>MTNQYSVKPQLVMFTGGRDSTLAACYLMLQGIPVHLWSGNSGCSLHRGILSHRVEEMKNRFGDLVVGHTVADISGAFRSIAIEALEQDILKYRKNLVLLGEKLAIHAHLVDFCRRNDINTINDGITHYQMEFPEQRLVAKTFLMEMMAQYDINYQSPVYEFAQSADDVKYRLLQLGISTKSLEGISIFADSFSTPSDDVVLAYLREKAPLAHNIVNFLAGETLNPP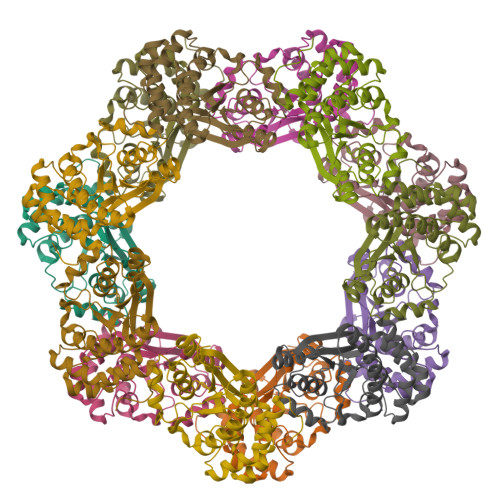VLNNSAAA[14x]> MKIAILSRDGTLYSCKRLREAAIQRGHLVEILDPLSCYMNINPAASSIHYKGRKLPHFDAVIPRIGTAITFYGTAALRQFEMLGSYPLNESVAIARARDK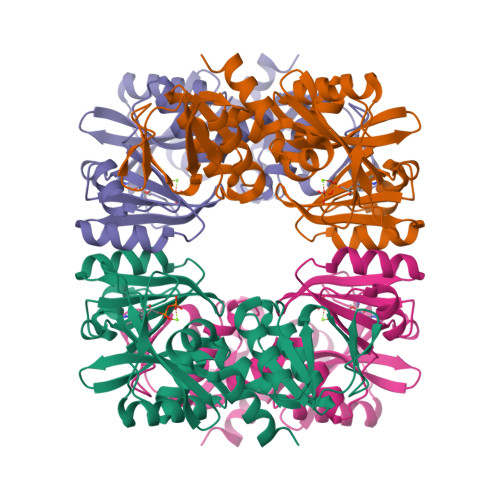LRSMQLLARQGIDLPVTGIAHSPDDTSDLIDMVGGAPLVVKLVEGTQGIGVVLAETRQAAESVIDAFRGLNAHILVQEYIKEAQGCDIRCLVVGDEVVAAIERRAKEGDFRSNLHRGGAASVASITPQEREIAIKAARTMALDVAGVDILRANRGPLVMEVNASPGLEGIEKTTGIDIAGKMIRWIERHATTEYCLKTGGGTLVPR>MGSMATLKAQHLAKSYKGRQVVRDVSMSIDSGQIVGLLGPNGAGKTTCFYMIVGLVQADQGVVRIDEQNVTHLPMHGRARAGIGYLPQEASIFRKLSVSDNIMAILETRSDLDRNGRKEALEGLLQEFHIHHIRDNLGMSLSGGERRRVEIARALASAPKFILLDEPFAGVDPISVGDIKQIIHHLKAKGIGILITDHNVRETLDICETAYIVNDGQLIAEGDAESILANDLVKEVYLGHEFRLKLHHHHHH[2x];> MGSMPKTLRQKLLLALIALLLIVAGYYWNVGLELFNEQPTRPGQDNTIDYYAENAHSLQYQEDGSLDYEMTAVKLEHQKATDITFVTTPDLLLFRGNVQPWHIQSARAEVGPKGKEVELIDDVRVARTDAKGQPSILTTTRLTVFPDKNYAQTEQAVKIDAANGVTTAVGMKAYLKDSRMHLLSNVRGQHEVR;> MGSMIVFRYLSREVLVTMSAVSAVLLVIIMSGRFIKYLAQAAQGLLDPGSLFLIMAFRIPGFLQLILPLGLFLGILLAYGRLYLESEMTVLSATGMSQKRLLGYTMAPALLVAILVAWLSLFLAPQGINQFALLLNKQDTLTEFDTLVPGRFQAMRDGTRVTYTEELSKDRGELAGIFISQKDLNSSNQERGISILVAEKGTQNIQADGSRYLILHNGYRYDGNPGQANYRAIQYDTYGVMLPKPEASSEVSERDAVPTADLFGSDNPRYQAELQWRLSTPLLVFVVTLLAVPLSRVNPRQGRFLKLLPAILLYMGYLALLIAVRGQLDKGKIPMAIGLWWVHGLFLAIGLLLFYWEPLRLKLASSRAGREVAHG;> MGSMVKLDRYIGVTVFVAILAVLGVILGLALLFAFIDELNDISASYGIGDALRFIFLTAPRRAYDMLPMAALIGCLVGLGTLASNSELTIMRAAGVSLSRIVWAVMKPMLVLMLAGILVGEYVAPWTENIAQSGRALAQGGGDSQSSKRGLWHRQGREYIHINAVQPNGVLYGVTRYRFDEQRGLESASFAKRARFETDHWQLEEVTTTLLHPREKRSEVVKLPTERWDAQLSPQLLNTVVMEPEALSISGLWQYIHYLADQGLNNNRYWLAFWTKVLQPLVTAALVLMAISFIFGPLRSVTLGQRIFTGVLVGFVFRIAQDLLGPSSLVFDFPPLLAVVIPASICALAGVWLLRRAG

The IM sub-complex comprises the ATP-binding cassette (ABC) transporter LptB2FGC, which extracts LPS from the IM and delivers it to the periplasmic components of the Lpt system. LptB2FGC is a type VI ABC transporter consisting of 5 subunits. The LptB cytoplasmic subunits form the nucleotide-binding domains (NBDs) that capture and hydrolyse ATP. LptF and LptG possess transmembrane helices that create a cavity and a translocation path for LPS, as well as a periplasmic β-jellyroll domain.

We also obtained two cryo-EM 3D reconstitutions of LptB2FGC at resolutions of 3.26 Å and 3.61 Å, respectively. These two structures were assigned as LptB2FGC-I and LptB2FGC-II. Structure alignment of these two structures gives rise to a root mean square deviation (RMSD) of 1.2 Å over 1324 Cα atoms and indicates the main difference between these two cryo-EM structures is in the β-jellyroll structures. These regions appear to perform a rigid body rotation motion toward the outer leaflet of IM, similarly to what we observed for LptB2FG. The TMD and NBD domains of LptB2FGC are similar to those of the LptB2FG structures and represent the resting state. In our LptB2FGC structures, the periplasmic β-jellyroll of LptC was clearly resolved and found to form a trimeric interface: LptC and LptF form the primary LPS transfer path, while a loop from LptG (residues 209–215) binds onto the N-terminal β-jellyroll of LptC (residues 60–69). Intriguingly, in contrast to previously documented LptB2FGC structures, the transmembrane helix of LptC remained unobservable in these maps, indicating its flexibility and a lack of engagement with LptF and LptG at Interface 1. This, in turn, results in an unobstructed entry point for LPS into the TMD cavity. Similar to LptB2FG, we identified four lipids in the transmembrane region of the form I conformation, which likely originate from nanodisc reconstitution. Our cryo-EM structures of P. aeruginosa LptB2FGC revealed a unique heterotrimeric interface between LptC, LptF, and LptG, with species-specific β-jellyroll contacts that likely underlie the failure of P. aeruginosa LptC to complement the E. coli system.>[2x]CPRFLKVKNWETEVVLTDTLHLKSTLETGCTEYICMGSIMH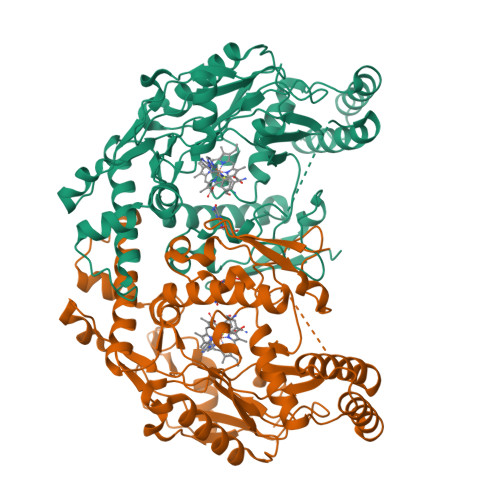PSQHARRPEDVATKDQLFPLAKEFIDQYYSSIKRFGSKAHMERLEEVNKEIDTTSTYQLKDTELIYGAKHAWRNASRCVGRIQWSKLQVFDARDCTTAHGMFNYICNHVKYATNKGNLRSAITIFPQRTDGKHDFRVWNSQLIRYAGYKQPDGSTLGDPANVQFTEICIQQGWKPPRGRFDVLPLLLQANGNDPELFQIPPELVLEVPIRHPKFEWFKDLGLKWYGLPAVSNMLLEIGGLEFSACPFSGWYMGTEIGVRDYCDNSRYNILEEVAKKMNLDMRKTSSLWKDQALVEINIAVLYSFQSDKVTIVDHHSATESFIKHMENEYRCRGGCPADWVWIVPPMSGSITPVFHQEMLNYRLTPSFEYQPDPWNTHVWKG> GAMGKVTHSIHIEKSDTAADTYGFSLSSVEEDGIRRLYVNSVKETGLASKKGLKAGDEILEINNRAADALNSSMME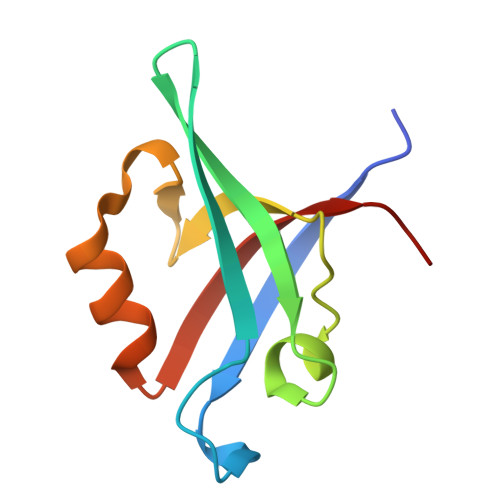DFFSQPSVGLLVRTYPEL>[3x]M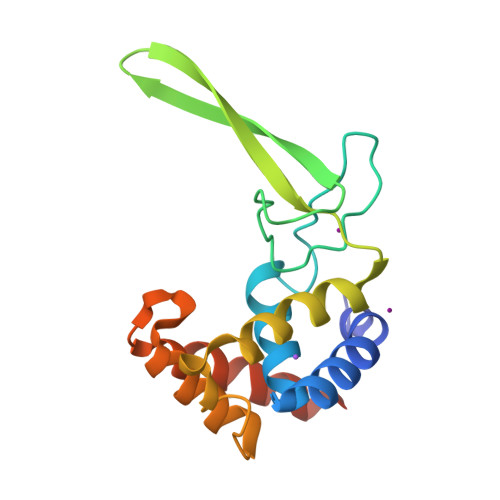DSKDFLARLSLPARLASEQSGVPHHLILAQAALESGWGQRQILRENGEPSYNVFGVKATASWKGPVTEITTTEYENGEAKKVKAKFRVYSSYLEALSDYVALLTRNPRYAAVTTAATAEQGAVALQNAGYATDPNYARKLTSMIQQLKAMSGSHHHHHH>[2x]MDNKTYEISSAEWEVMNIIWMKKYASANNIIEEIQMQKDWSPKTIRTLITRLYKKGFIDRKKDNKIFQYYSLVEESDIKYKTSKNFINKVYKGGFNSLVLNFVEKEDLSQDE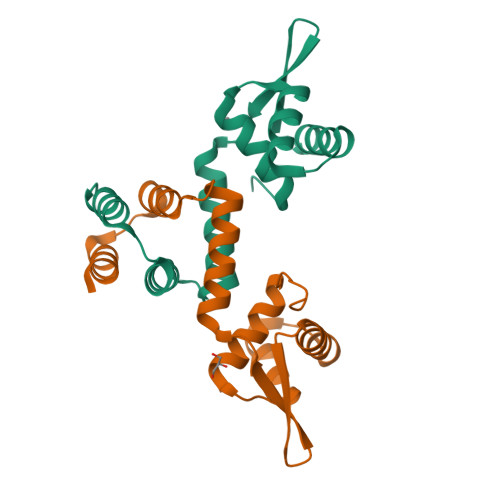IEELRNILNKK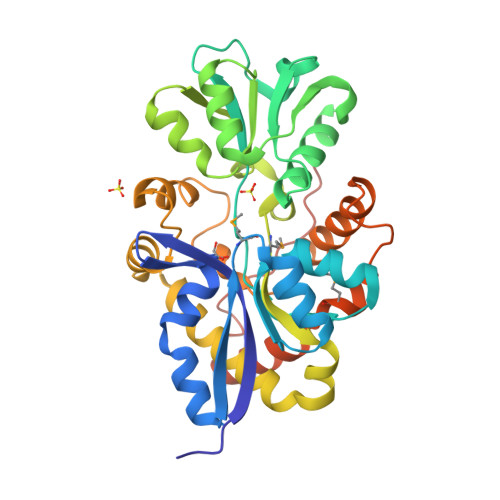> MVEDLKVVRIASVATNVGGKTVYAGSASLVVNGAFPEELRKQGIKVEWVPAAMASVGPVINEGFASGKIDFGIYGDLPPIILNASKPTVQLVAPWGTTSNSYLVVPKNSTAKSIKDLKGKKIALHRGRPWELAFSNLLQSEGLTFKDFKIVNVNPQVGAAALASGTVDGFFSLFDSYILEDRGVGKIIWSTKTAPVDWKLMGGVWARNDFVKQNPEITQAIVTAYLKSVHWVAQDENKETYIREYSNKIYPESVNRREYDQDNVSWRQRWSPLYDVALQEHYRKAVAYAQASGLTRTQADVQQMLNPHFVATALKELKLEGFWTPNAENLYFQSHHHHHHWSHPQFEK>TGGGGT[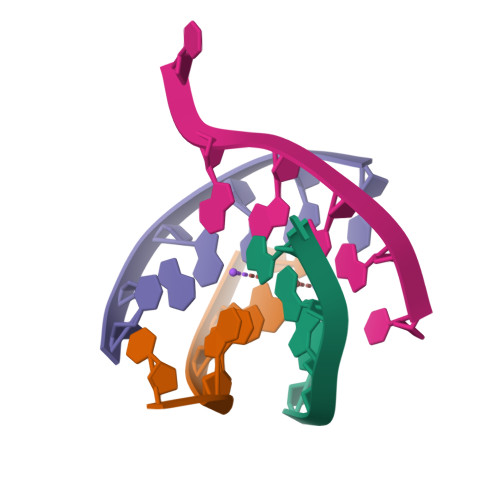12x]> AQAFVDATWPQAAKA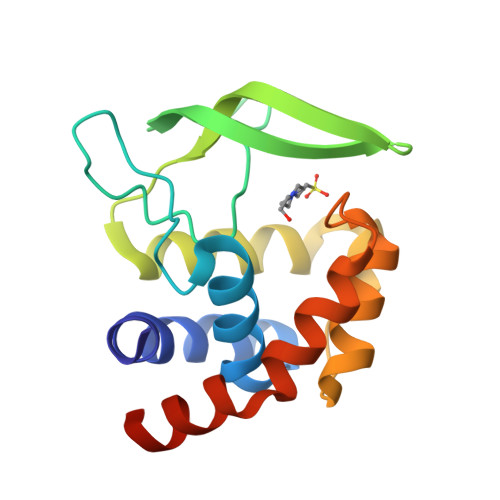AQSLGVPAHFLVAQAALETGWGKSQIRNKDGTPSYNLFNIKAGSNWTGKVVEARTVEYENGQRKVRVERFRAYDSYEQAFQDYADLVGNSPRYAKVAGKTDGHAFARALQEGGYATDPSYADKLARVINGNALRQRLMHHHHHHHH>MGGSSHHHHHHSSGLVPRGSGGLTHRKFGGYGGSPFSGLSSIAVRSGSYLDAIIIDGVHHGGYGGNLSPTFTFGSGEYISNMTIRSGDYIDNISFETNMGRRFGPYGGYGGSANTLSNVKVIQINGSAGDYLDS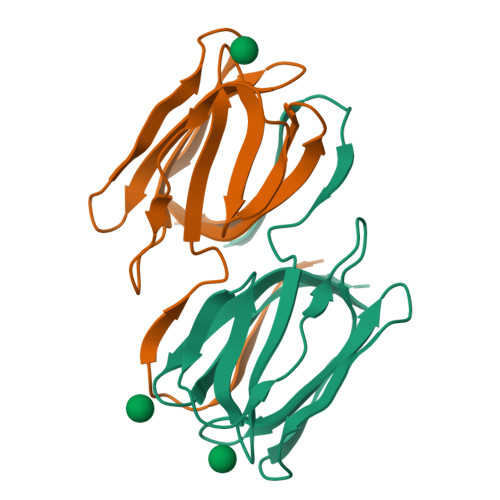LDIYYEQY[2x]>ETWWYNPSIVVHPHWREFDQVPDAVYYSLGIFIGICGIIGCGGNGIVIYLFTKTKSLQTPANMFIINLAFSDFTFSLVNGFPLMTISCFLKKWIFGFAACKVYGFIGGIFGFMSIMTMAMISIDRYNVIGRPMAASKKMSHRRAFIMIIFVWLWSVLWAIGPIFGWGAYTLEGVLCNCSFDYISRDSTTRSNILCMFILGFFGPILIIFFCYFNIVMSVSNHEKEMAAMAKRLNAKELRKAQAGANAEMRLAKISIV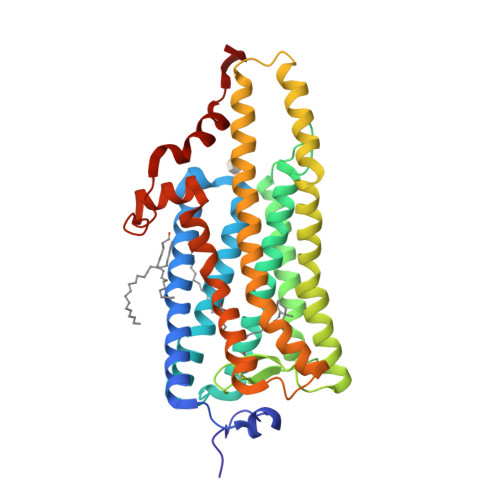IVSQFLLSWSPYAVVALLAQFGPLEWVTPYAAQLPVMFAKASAIHNPMIYSVSHPKFREAISQTFPWVLTCCQFDDKETEDDKDAETEIPAGE[2x]> S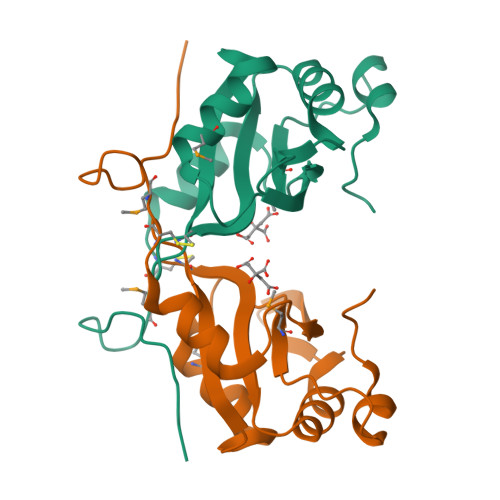LNPDLNLQRYTPTVEKHASDRNSVDYAQIASGIDTRTTVMIKNIPNKFTQQMLRDYIDVTNKGTYDFLYLRIDFVNKCNVGYAFINFIEPQSIITFGKARVGTQWNVFHSEKICDISYANIQGKDRLIEKFRNSCVMDENPAYRPKIFVSHG Many NLR proteins nucleate the “inflammasome”—a large macromolecular complex that triggers inflammatory cell death and cytokine secretion in response to microbial or danger-associated ligands. Like many other supramolecular assemblies in the human innate immune system, the inflammasome complex relies on homotypic and heterotypic interactions between the death domains (DDs) to initiate, amplify, and propagate pyroptotic signaling. Inflammasome sensor NLRs can be grouped into two categories based on their DDs: PYRIN domain (PYD) and caspase activation and recruitment domain (CARD), both domains were found to form filamentous complexes to initiate the inflammasome formation. Extending this analysis, we also found that specific type II interface motifs directly dictate the compatibility of heterotypic pairwise CARD-CARD interactions among NLRP1, CARD8, NLRC4, ASC, and CASP1.

To test this, we solved the structures of recombinant NLRP1-CARD and CARD8-CARD filaments using cryo-EM, both at 3.7 Å with Gold standard FSC = 0.143, without masking. Similar to NLRP1-CARD, recombinant CARD8-CARD also formed ~8 nm-wide filaments, but these filaments are more rigid and adopt a single conformation. NLRP1-CARD and CARD8-CARD filaments display similar helical parameters (5.36 Å and −100.8 degree for NLRP1, and 5.409 Å and −99.16 degree for CARD8), suggesting a similar mode of assembly from the respective monomers. Despite near-identical helical parameters, NLRP1-CARD and CARD8-CARD filaments have remarkably different surface charge distributions, that are not suggested by their monomer structures alone. By contrast, in CARD8-CARD filaments, the positively charged patches on the monomer are mostly buried inside the filamentous oligomer, exposing a predominantly negative surface. In contrast, the CARD8 Type IIb surface is partially negatively charged (Tyr531, Tyr527, and Asp525), whereas the Type IIa surface is positive (Lys508, Lys509, and Leu512). Hence, CARD8-CARD is structurally compatible with CASP1-CARD but not ASC-CARD. In agreement with the structural predictions, CARD8-CARD, but not NLRP1-CARD, preferentially stimulated CASP1-CARD oligomerization, as demonstrated by the appearance of slower migrating bands on native gels (lanes 2 and 3 vs. 4 and 5), whereas the reverse was true for ASC-CARD oligomerization (lanes 2 and 3 vs. lanes 4 and 5). We further corroborated that CARD8 is the first human inflammasome sensor that is unable to engage ASC as an amplifier. In contrast, CARD8-dependent pyroptosis was not abrogated in ASC (PYCARD) KO keratinocytes (blue bars).

>GPGMAAFVKENHRQLQARMGDLKGVLDDLQDNEVLTENEKELVEQEKTRQSKNEALLSMVEKKGDLALDVLFRSISERDPYLVSYLRQQNL[12x]> GSLQVTVRDAINQGMDEELERDEKVFLLGEEVAQYDGAYKVSRGLWKKYGDKRIIDTPISEMGFAGIAVGAAMAGLRPICEFMTFNFSMQAIDQVINSAAKTYYMSGGLQPVPIVFRGPNGASAGVAAQHSQCFAAWYGHCPGLKVVSPWNSEDAKGLIKSAIRDNNPVVVLENELMYGVPFEFPPEAQSKDFLIPIGKAKIERQGTHITVVSHSRPVGHCLEAAAVLSKEGVECEVINMRTIRPMDMETIEASVMKTNHLVTVEGGWPQFGVGAEICAR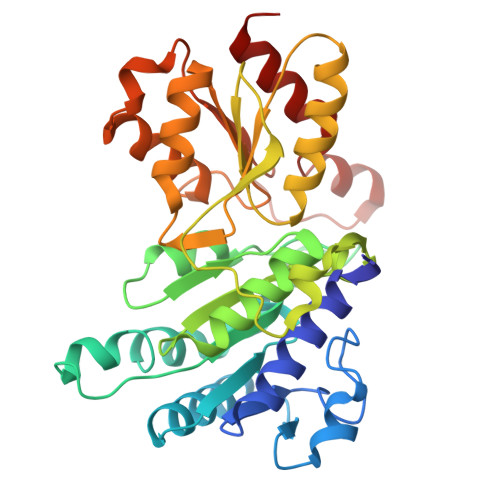IMEGPAFNFLDAPAVRVTGADVPMPYAKILEDNSIPQVKDIIFAIKKTLNI>[6x]MFGKRDSSASGDPKAPPPAPAGGATIATRPQRVEPVAAPEPKAPAPKVSGPAPKPTVGLEQLRAAQGQPQTANIVREQSDYYHATKTTIFNALLNTIDLSQLAQLDLKQAGEEIRDIVAELVAIKNVSMSVAEQEHLVQDIINDVLGYGPLEPLLARDDIADIMVNGAHRVFIEVGGKVQLTNVRFRDNLQLMNICQRI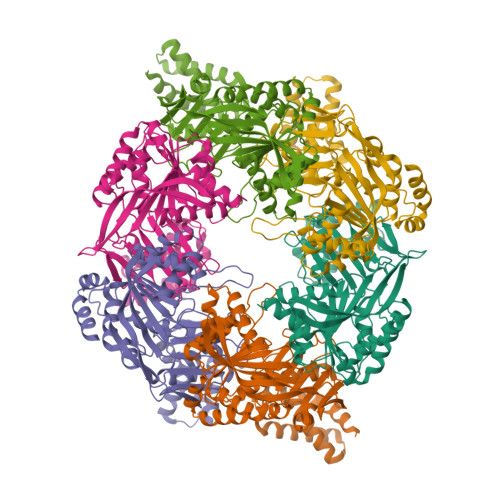VSQVGRRVDESSPICDARLPDGSRVNVIAPPLALDGPTLTIRKFKKDKLTMKNLVEFASISPEGARVLGVIGACRCNLVISGGTGSGKTTLLNTMTAFIDPTERVVTCEDAAELQLQQPHVVRLETRPPNLEGSGAVTMRDLVKNCLRMRPERIIVGEVRGPEAFDLLQAMNTGHDGSMGTLHANSPREAISRIESMITMGGYGLPSKTIKEMIVGSVDVIIQAARLRDGSRRITHITEVVGLEGDVIVTQDLFVYEITGEDEHGKVVGKHRSTGIARPRFWDRARYYGLERELAEALDAAE> EGTGSANRVRR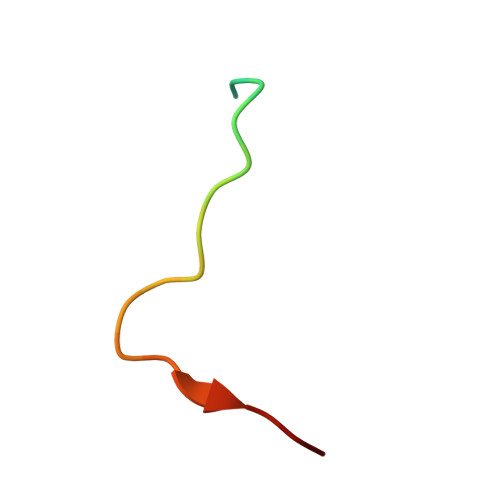PPREGHIYMAS> GSPEFMHTINEEERREFIKHINSVLAGDPDVGSRVPINTETFEFFDQCKDGLILSKLINDSVPDTIDERVLNKQRNNKPLDNFKCIENNNVVIN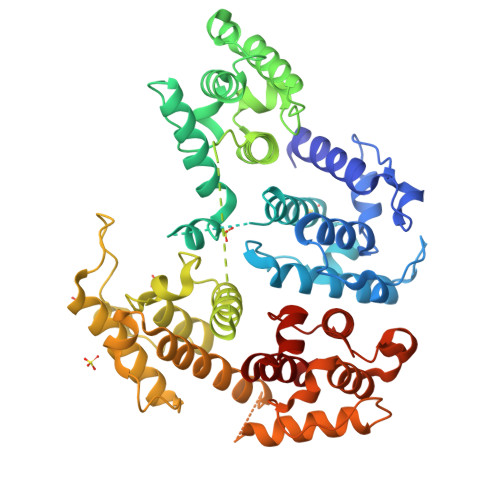SAKAMGGISITNIGAGDILEGREHLILGLVWQIIRRGLLGKIDITLHPELYRLLEEDETLDQFLRLPPEKILLRWFNYHLKAANWPRTVSNFSKDVSDGENYTVLLNQLAPELCSRAPLQTTDVLQRAEQVLQNAEKLDCRKYLTPTAMVAGNPKLNLAFVAHLFNTHPGLEPLNEEEKPEIEPFDAEGEREARVFTLWLNSLDVTPSIHDFFNNLRDGLILLQAYDKITPNTVNWKKVNKAPASGDEMMRFKAVENCNYAVDLGKNQGFSLVGIQGADITDGSRTLTLALVWQMMRMNITKTLHSLSRGGKTLSDSDMVAWANSMAAKGGKGSQIRSFRDPSISTGVFVLDVLHGIKSEYVDYNLVTDGSTEELAIQNARLAISIARKLGAVIFILPEDIVAVRPRLVLHFIGSLMAV>[2x]MSALNPALRFRDFIQVLKNEGDLIEITTEVDPNLEVGAITRKVYEEKLPAPLFNNLKGASKNLFNILGCPGGLRSKKGNDHARIALHLGLDSQTPMKKIIDYLLEAKTKKPIPPHEVPASGA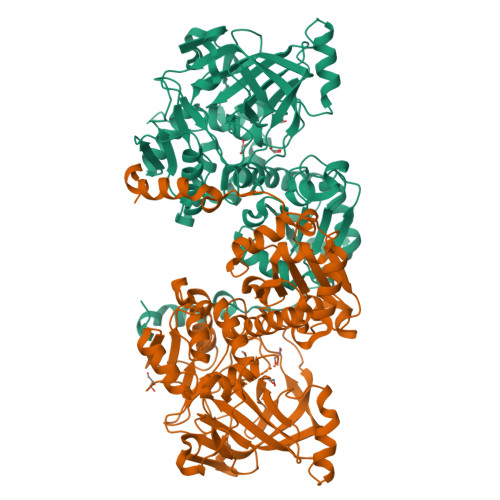PCKENLLSGDEIDLTSLPVPLLHHGDGGKYIQTYGMWVLQTPDKSWTNWSIARGMVVDDKHITGLVINPQHIRQVADAWAAIGKGDKIPFALCFGVPPAAILVSSMPIPEGATESDYIGALLGESLPVVKCETNDLMVPATSEIVFEGTLDLNDLVPEGPFGEMHGYVFPGQGHPCPLYTVNAITYRNNAILPVSNPGLCTDETHTLIGGLVSAEAKQLAIEHGVPILDAFTPYEAQALWLALKVDLKKLQALKTNPKEFSKKVGDIYFRSKVGFIIHEIILVGDDIDIFDFRKVIWAYTTRHTPVDDQYYFDDVKAFALAPFVSQSPRIKTLKGGKCVTNCIFPQQYERDVDFVTCNFDGYPEEIKDKVLQNWSAYGYK> AVRHLTGSVTRTQGLRFAVVVARFNEIITRPLLEGALGTFKNYSVQDEDIDVVWVPGCFEIGAVATRLGKSGKYHAIICIGAVIRGD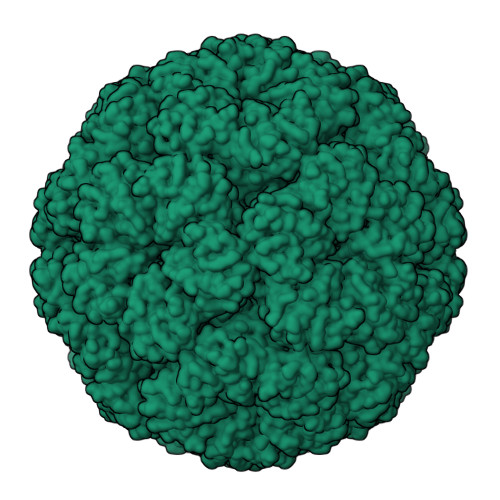TTHYDAVANSAASGVLSAGLNSGVPCIFGVLTCEDMDQAINRAGGKSGNKGAEAALTAIEMASLFEHHLQ> XVAEIQLMHQRAKWLNSLERVEW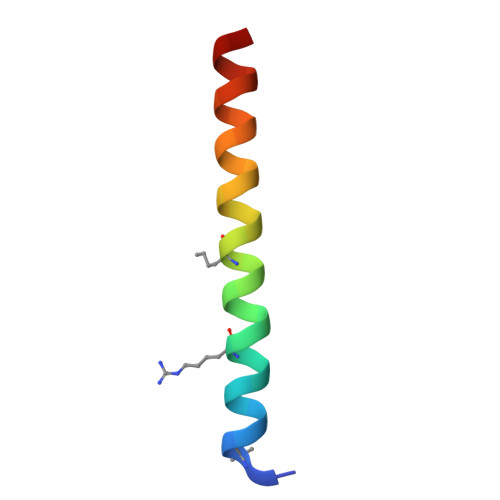LRKKLQDVHNYX>[2x]SNAGEVVDCHLSDMLQQLHSVNASKPSERGLVRQEEAEDPACIPIFWVSKWVDYSDKYGLGYQLCDNSVGVLFNDSTRLILYNDGDSLQYIERDGTESYLTVSSHPNSLMKKI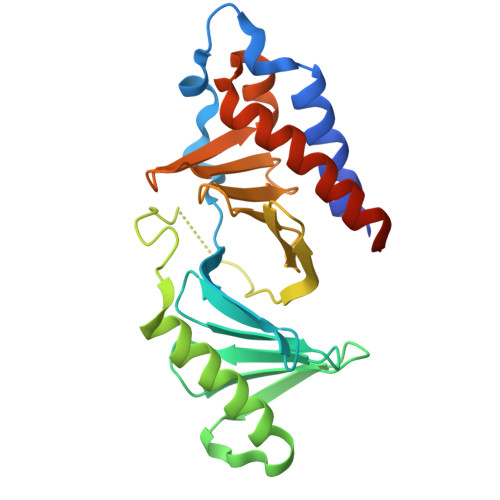TLLKYFRNYMSEHLLKAGANITPREGDELARLPYLRTWFRTRSAIILHLSNGSVQINFFQDHTKLILCPLMAAVTYIDEKRDFRTYRLSLLEEYGCCKELASRLRYARTMVDKLLSSRSASNRLKAS> HMSLSVANSTYETTALNSQKSSTDQPNSGSKSGQTLDLVNLGVAANFAILSKT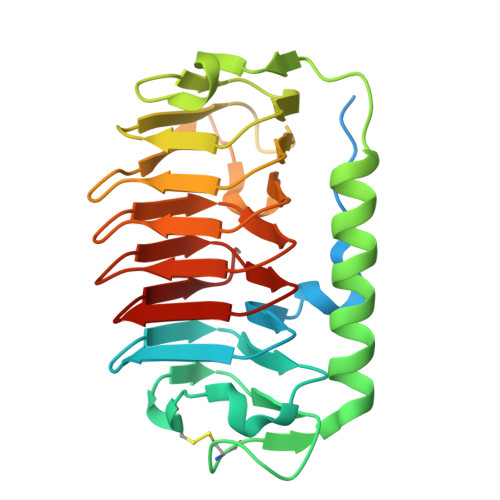GITDVYKSAITGDVGACPITGAAILLKCDEVTGTIFSVDAAGPACKITDASRCTTAVGDMQIAYDNAAGRLNPDFLNLGAGTIGGKTLTPGLYKWTSTLNIPTDITISGSSTDVWIFQVAGNLNMSSAVRITLAGGAQAKNIFWQTAGAVTLGSTSHFEGNILSQTGINMKTAASINGRMMAQTAVTLQMNTVTIPQ> SPTVEACGYSDRIIQITRGDSTITSQDVANAIVAYGVWPHYLSSKDASAIDKPSQPDTSSNRFYTLRSVTWSSSSKGWWWKLPDALKDMGIFGENMFYHYLGRSGYTIHVQCNASKFHQGTLIVALIPEHQIASALHGNVNVGYNYTHPGETGREVKAETRLNPDLQPTEEYWLNFDGTLLGNITIFPHQFINLRSNNSATIIAPYVNAVPMDSMRSHNNWS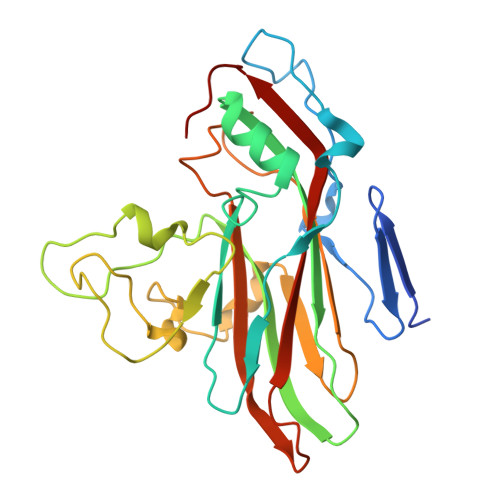LVIIPICPLETSSAINTIPITISISPMCAEFSGARAKRQ> MKKAISCVFLISALILSSFQVPVQGQAMSKTTSAAGNSVSYDGERRVNFNENWRFQRETNGSIAGAQNPGFDDSSWRKLNLPHDWSIELDFNKNSLATHEGGYLDGGIGWYRKTFTIPESMKGKRISLDFDGVYMNSTTYLNGEVLGTYPFGYNAFSYDISDKLYKDGRANVLVVKVNNTQPSSRWYSGSGIYRNVYLTVTDPIHVARYGTFVTTPNLEKSIKEDRADVNIKTKISNDAAEAKQVKIKSTIYDGAGNTVQTVETEEKTAAAGTVTPFEQNTVIKQPKLWSIDKPYRYNLVTEVIVGGQTVDTYETKFGVRYFKFDENEGFSLNGEYMKLHGVSMHHDLGALGAATNARGVERQMQIMKDMGVNAIRVTHNPASPELLEAANKLGLFIIEEAFDSWAQSKKPYDYGRFFNAWAEHDIKEMVDRGKNEPAIIMWSIGNEIYDTTNAAGVETARNLVGWVKEIDTTRPTTIGEDKTRGDKVNVTPINSYIKEIFNIVDVVGLNYSENNYDGYHKQNPSWKLYGSETSSATRSRGVYTHPYQYNQSTKYADLQQSSYDNDYVGWGRTAEDAWKYDRDLKHIAGQFIWTGFDYIGEPTPYYNSYPAKSSYFGAVDTAGFPKDIFYYYQSQWKKEPMVHLLPHWNWKEGEKVRVLAYTNASKVELVLNGESLGEKNYDNKQTSWGAPYKETKDGKTYLEWAVPFKPGKLEAVAKDENGKVIARDQVVTAGEPASVRLTADRKVVKADGTDLSFITADIVDSKGIVVPDADHLITFNVTGQGELAGVDNGNASSVERYKDNKRKAFSG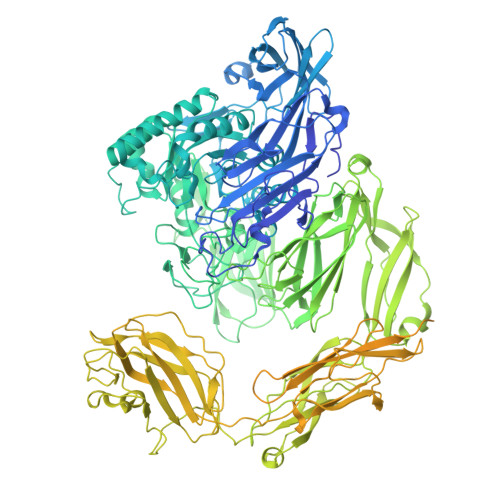KALAIVQSSKLSGKITVHASVAGLSSDSTSVFTVTPADHDKKIVAGIDDVNLTVDVNEAPKLPSEIKVYYSDESAAAKNVTWDEVDPKQYSTVGEFTVEGSVEGTSLKAKAFVIVKGIVAVKPYSTATKVGVQPVLPEKATLLYSDGTTKGATVTWDEIPEDKLAKEGRFTVEGSVEGTDLKANVYVRVTNEVKSVNIMLQEQGSAYPKLEATFTNPADNLQHLNDGIKSYTNNPVNRWTNWTRTPRDAGDSITVNFGKKHVINNLDLFVFTDSGTVVPEKAEVQYWDGTAWKDVENLTQPSPYVVEKNELTFDAVATEKLKFHLTPSVKGKFLALTEAEVYADQIVMGETAKLQSITVNGKALEGFDHAKKNYELVLPYGSELPKIEAAAADNATVTILPAFSYPGTAKLFVTSEDGKVTTEYSIGVSTEEPKLVSAELSADKTNVMEDDIIDLKVIGLFESKEKIDVTDSQPTYEFDQQIIKIEGNKLYALETGNVKVKVTVTYKGVSVTTPALEFTIAKNPAPKYITSLEPVTVVVKKGEAPELPATVVAHYNRGIPRDVKVKWERINPSKYQQLGEFTVSGMVEGTDIKAQAKVIVKGAVAVEDIRMAVLLKQMPQLPGKVTVYYSDGAEEQRAVKWEEIPQEELENVGEFKVKGDVNGVKLKATATIRVTDEVGGEQNISRAKNGYEYPKAEASFTNNGPGSSDRIEAINDDVISYEANPHNRWTNWQPVPRAGDWVSITFGDYEPTEYDVDSMEIHWFADHGTSYPERFQIEYKSGDSWKEVTSLKSDPASPALGKANVYSFDRVKTSAIRVKMTAQAGKSLAITELKVFSKWPKAGTEPEVTDIKVGGKSILEDFEQKGDHYEVTIDAGDANVMPKINVKAKDQTSITIVPAVTSPSTAKVIAKSEDGKKVKVYSIHYK> SNAMVDSYDDSLDGEKSKTQVKRELHALVDLGERLTTLKADVLAKLPLTDALRKALAEAPKHTANIARKRHILFIGKLMRDQDQEAILVLLDQLD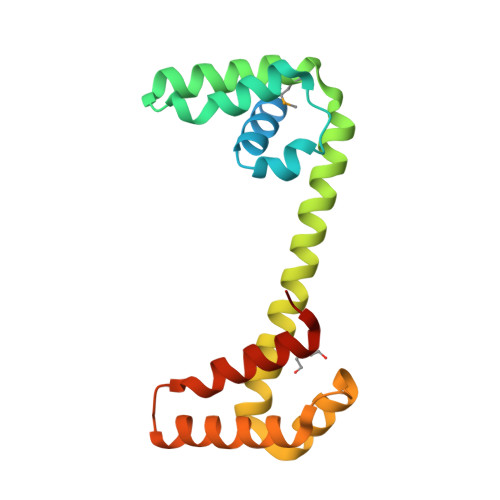ASTRQYNERFHNLERWRDRLIAGDDADLEKFVIEYPDADRQQLRSLIRQAQHEVARNKPPATSRKIFKYIRELDELQRGLR>[2x]GSGSGMDEIVKVLSQHDRILVVGHIMPDGDCVSSVLSLTLGLEKLGKEVKAAVDYKIPYVFEKFPYIDKIEENPNFDPELLVVVNA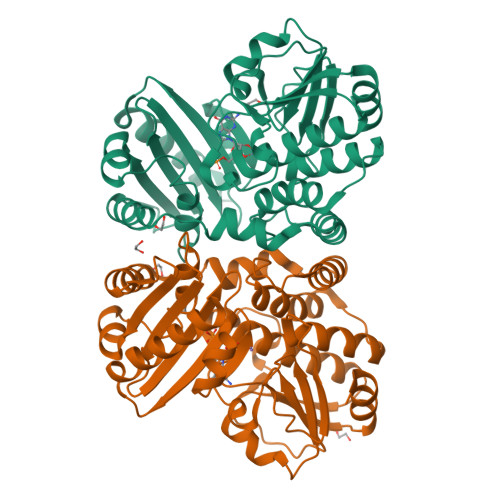SSPDRIGKFQDLLDKVPSVVIDHHSTNTNFGNWNWVDPSFAATAQMIFRINKALGVEYDSNLATLNYLGIATNTGFFRHSNADVRVFEDAYKLVKMGADAHFVAKEILENKRFEQFKLFAEVLERLQLLENGKIAYSYIDYDTYLRHNCTDEDSAGFVGELRSIRGVEVAVLFMEFPRGKIHVSMRSKDWFNVNEVAFELGGGGHPRAAGVTFEGKKIEEVIPRVINHLLKKFKEGVESESEKIPEGDVLGG> MSKKKFVIVSILTILLVQAIYFVEKYHTSEDKSTSNTSSTPPQTTLSTTKVLKIRYPDDGEWPGAPIDKDGDGNPEFYIEINLWNILNATGFAEMTYNLTSGVLHYVQQLDNIVLRDRSNWVHGYPEIFYGNKPWNANYATDGPIPLPSKVSNLTDF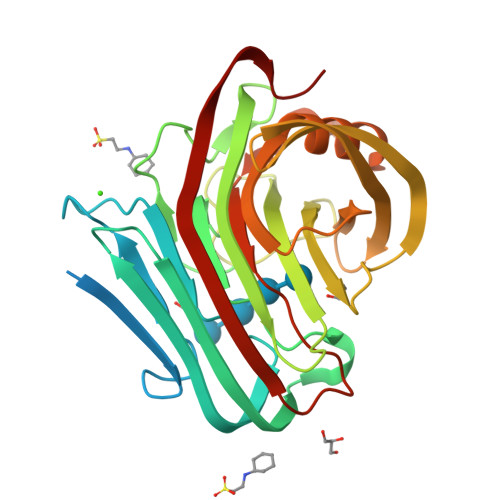YLTISYKLEPKNGLPINFAIESWLTREAWRTTGINSDEQEVMIWIYYDGLQPAGSKVKEIVVPIIVNGTPVNATFEVWKANIGWEYVAFRIKTPIKEGTVTIPYGAFISVAANISSLPNYTELYLEDVEIGTEFGTPSTTSAHLEWWITNITLTPLDRPLIS> MKQFTKCELSQLLKDIDGYGGIALPELICTMFHTSGYDTQAIVENNESTEYGLFQISNKLW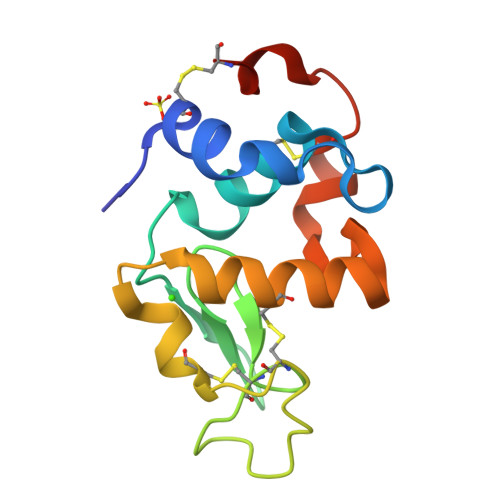CKSSQVPQSRNICDISCDKFLDDDITDDIMCAKKILDIKGIDYWLAHKALCTEKLEQWLCEKL>[3x]MPMISCDMRYGRTDEQKRALSAGLLRVISEATGEPRENIFFVIREGSGINFVQHGEHLPDYVPGNANDKALIAKLK;>PFIECHIATGLSVARKQQLIRDVIDVTNKSIGSDPKI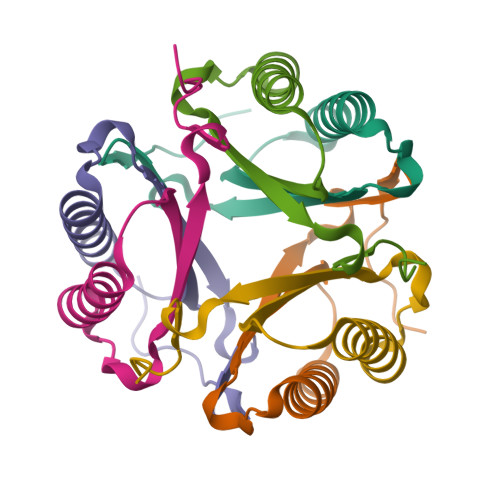INVLLVEHAEANMSISGRIHGEAASTERTPAVS[3x]> MSESLSWMQTGDTLALSGELDQDVLLPLWEMREEAVKGITCIDLSRVSRVDTGGLALLLHLIDLAKKQGNNVTLQ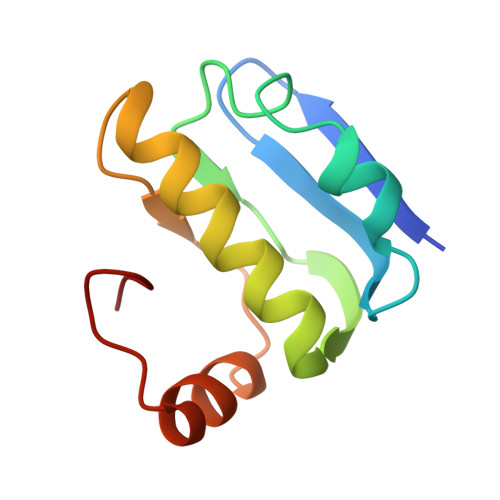GVNDKVYTLAKLYNLPADVLPR BIOTIN-D-SULFOXIDE | C10 H16 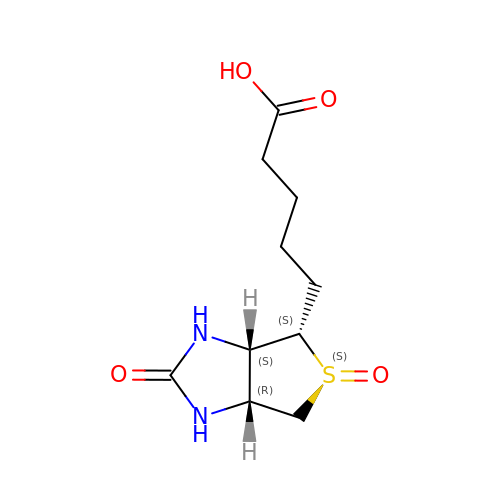N2 O4 S | KCSKCIQYNAOBNQ-OKPRWBIXSA-N> HHHHHHVSQVHRILNCRGTRIHAVADSPPDQQGPLVVLLHGFPESWYSWRHQIPALAGAGYRVVAIDQRGYGRSSKYRVQKAYRIKELVGDVVGVLDSYGAEQAFVVGHDWGAPVAWTFAWLHPDRCAGVVGISVPFAGRGVIGLPGSPFGERRPSDYHLELAGPGRVWYQDYFAVQDGIITEIEEDLRGWLLGLTYTVSGE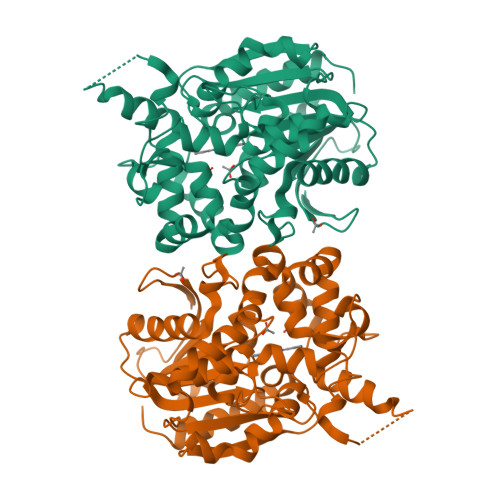GMMAATKAAVDAGVDLESMDPIDVIRAGPLCMAEGARLKDAFVYPETMPAWFTEADLDFYTGEFERSGFGGPLSFYHNIDNDWHDLADQQGKPLTPPALFIGGQYDVGTIWGAQAIERAHEVMPNYRGTHMIADVGHWIQQEAPEETNRLLLDFLGGLRP>MTSPVIGTPWKKLNAPVSEEALEGVDKYWRVANYLSIGQIYLRSNPLMKEPFTREDVKHRLVGHWGTTPGLNFLIGHINRFIADHGQNTVIIMGPGHGGPAGTSQSYLDGTYTETFPKITKDEAGLQKFFRQFSYPGGIPSHFAPETPGSIHEGGELGYALSHAYGAIMDNPSLFVPAIVGDGEAETGPLATGWQSNKLVNPRTDGIVLPILHLNGYKIANPTILSRISDEELHEFFHGMGYEPYEFVAGFDDEDHMSIHRRFAELWETIWDEICDIKATAQTDNVHRPFYPMLIFRTPKGWTCPKYIDGKKTEGSWRSHQVPLASARDTEAHFEVLKNWLESYKPEELFDANGAVKDDVLAFMPKGELRIGANPNANGGVIRNDLKLPNLEDYEVKEVAEYGHGWGQLEATRTLGAYTRDIIKNNPRDFRIFGPDETASNRLQASYEVTNKQWDAGYISDEVDEHMHVSGQVVEQLSEHQMEGFLEAYLLTGRHGIWSSYESFVHVIDSMLNQHAKWLEATVREIPWRKPIASMNLLVSSHVWRQDHNGFSHQDPGVTSVLLNKCFHNDHVIGIYFATDANMLLAIAEKCYKSTNKINAIIAGKQPAATWLTLDEARAELEKGAAAWDWASTAKNNDEAEVVLAAAGDVPTQEIMAASDKLKELGVKFKVVNVADLLSLQSAKENDEALTDEEFADIFTADKPVLFAYHSYAHDVRGLIYDRPNHDNFNVHGYEEEGSTTTPYDMVRVNRIDRYELTAEALRMIDADKYADKIDELEKFRDEAFQFAVDNGYDHPDYTDWVYSGVNTDKKGAVTATAATAGDNE[8x]

Phosphoketolase (XPK) belongs to the transketolase family, a member of thiamine pyrophosphate (TPP)-dependent enzyme superfamily. It converts F6P, xylulose-5-phosphate (Xu5P) or sedoheptulose-7-phosphate (S7P), which are intermediates in RuBP regeneration, to produce acetyl phosphate (AcP) and C3, C4 or C5 sugar phosphates. XPK is an enzyme present in many microorganisms, primarily involved in substrate-level phosphorylation to produce AcP.

On the other hand, Bifidobacterium longum XPK showed no inhibition by ATP. Of note, while the dimer–dimer interface in the SeXPK dodecamer involves residues near the C terminus, the B. longum XPK octamer involves residues near the N terminus. As the donut-shape or four-leaf clover shape-like particles or two-dimensional (2D) class average images were not in perfect symmetry, we further examined whether the assigned symmetries were pseudosymmetry. Some relative random motions were observed between different dimers in both SeXPK dodecamer and B. longum octamer assemblies, suggesting the likelihood of pseudosymmetry in these structures. Comparison between the C-terminal interfaces of free SeXPK and free B. longum XPK structures provides a structural basis for the lack of ATP inhibition in B. longum XPK.>RDHRKIGKQLDLYHMQEEAPGMVFWHNDGWTIFRELEVFVRSKLKEYQYQEVKGPFMMDRVLWEKTGHWDNYKDAMFTTSSENREYCIKPMNCPGHVQIFNQGLKSYRDLPLRMAEFGSCHRNEPSGSLHGLMRVRGFTQDDAHIFCTEEQIRDEVNGCIRLVYDMYSTFGFEKIVVKLSTRPEKRIGSDEMWDRAEADLAVALEENNIPFEYQLGEGAFYGPKIEFTLYDCLDRAWQCGTVQLDFSLPSRLSASYVGEDNERKVPVMIHRAILGSMERFIGILTEEFAGFFPTW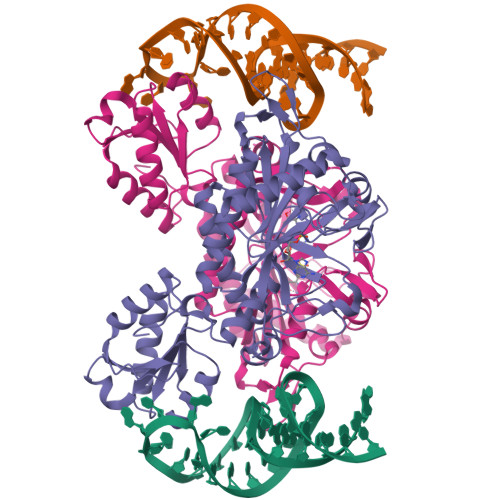LAPVQVVIMNITDSQSEYVNELTQKLSNAGIRVKADLRNEKIGFKIREHTLRRVPYMLVCGDKEVESGKVAVRTRRGKDLGSMDVNEVIEKLQQEIRSRSLKQLEE[8x]>GAMAEKPPKELVNEWSLKIRKEMRVVDRQIRDIQREEEKVKRSVKDAAKKGQKDVCIVLAKEMIRSRKAVSKLYASKAHMNSVLMGMKNQLAVLRVAGSLQKSTEVMKAMQSLVKIPEIQATMRELSKEM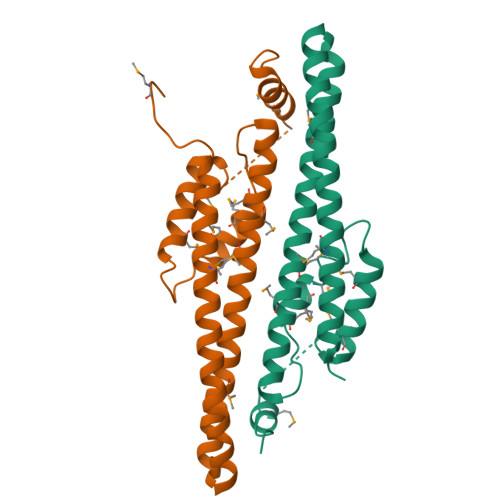MKAGIIEEMLEDTFESMDDQEEMEEEAEMEIDRILFEITAGALGKAPSK[4x]TrmD (tRNA-(N(1)G37) methyltransferase) is an essential tRNA modification enzyme in bacteria that prevents +1 errors in the reading frame during protein translation and represents an attractive potential target for the development of new antibiotics. TrmD belongs to a distinct class of S-adenosyl-l-methionine (SAM)-dependent methyltransferases known as the SpoU-TrmD (SPOUT) RNA methyltransferase superfamily or Class IV methyltransferases. Each non-crystallographic 2-fold symmetry-related protomer of TrmD interacts in an antiparallel manner and consists of two domains: a larger N-terminal domain spanning residues 1–161 and a smaller C-terminal helical domain (177–242) connected by a flexible inter-domain linker. The SAM binding region of TrmD is located at the base of the N-terminal domain and consists of a deep trefoil knot architecture, made of three distinct untwisted loop regions.

Structure-guided elaboration of the merged compound AW1 (Kd 0.11 mM, LE 0.36, IC50 0.23 mM) was performed, initially utilizing the indole nitrogen as a vector for growth. The addition of a 2-picolyl moiety successfully increased the affinity of AW1 by an order of magnitude in compound AW2 (Kd 12 μM, LE 0.30, IC50 33 μM). The methylene linker attached to the indole nitrogen of AW2 allowed the added pyridyl ring to occupy the region defined by Pro85, Glu112, Val137, Arg154 and Glu180. The affinity of AW2 was further improved by the addition of a nitrile group on the 4-position of its pyrazole ring, extending into the narrow space between residues 83PTP85 of the cover loop and 131VSI133 of the bottom loop respectively. AW3 (Kd 0.50 μM, LE 0.36, IC50 0.31 μM) was a significant improvement on AW2, with the addition of two heavy atoms affording a 25-fold decrease in Kd (12–0.50 μM), increasing the ligand efficiency to the level of the original merged compound AW1 (0.36), and a 100-fold decrease in IC50 (33 to 0.31 μM).

>[2x]GSMKIDVVTIFPEYLQPVRQSLPGKAIDAGLVDVAVHDLRRWTHDVHKSVDDSPYGGGPGMVMKPTVWGDALDEICTSETLLVVPTPAGYPFTQETAWQWSTEDHLVIACGRYEGIDQRVADDAATRMRVREVSIGDYVLNGGEAAALVIIEAVLRLVPGVLGNALSAQEDSHSEGMASLLEGPSYTRPPSWRGMDVPPVLLSGDHAKIAAWRAEQSRQRTIERRPDLLGFDSPTGEHGGDGLS> MSSRYRELIAIFGEFLEENDFHVRISMDRVGEVKTLFSAKTIPVESETEAAIEVVTIEAARRRDALRRTCNAVLRTRHSDQHVDVGTIVADEEERLAWKFLIGALAAKNSEILPVVEAELLLAAVEYHYATARPELCDMFVHLSASEMFFIDGDSLFMAALSPQSVDWDLIQPLHVIYNAQKLLYDMHCRGARFHVVFFDSLLWIWESAPAKLFMRENLRKTLMSLSENDAKVGLSISNFSSYYSEAFETYVKQWEPEFILMSDGEQLGRLNPLQAFFVRPSAANNTHDSRRKANYTDADEANPYRLRRQYRSIVEDEAVGDKAALYYRCIHLWAATRRLKVAYSSRIIYKENAMVVFTVRVDGASFERAVTIESDVQALAQSMEHEVQLPAISSASLGLLDEEDLSCRERVVYAALHAYLRASARSEQEHQLCQALAITTYITGYLNKEARAQQVRPNPILAGFLNEISPFLLAVWRHADCTNGNGQEFDLIDGHLFSAVSQQLRTASVSELFDEYGVEDIESTWGVLDDQGSADIVNAPLSYLPVIDSVDVEKLQPYPLITHELVERLAKGFGISTHRADAPYPTDFGAANELAGWDITTPFDRLNDVIDAEGDAIAKSMMTEKEAKNVQEYYKKFVRNALKQAQSMGISGFAAHELAMVCSDNDSDDDAGGNSANNKTAGAKKVNKEHAGQRNKKERSKEDEIRERSNVIAATATVAEWHKQMNHLLHAVDMSHGRTTNRDRDESINTIMAAIKRLSQEKFGKNFDPGYTLGGSTNTAVPLKLEMWRLLVAASQLREVEFAFAMEDPALKDSKGASKKKDSKSEYKMLYGFHVINQFVEREAVKGNHWGQLDPLRKAKPDMTIVEARSYLRWVYLSFVEMHIQLKLKCRVVKLQLENWRAERERARLAQESPKIALGIPLFLYCHHHVLAVIRDEGPRMSSEDIDTVRSALKHFDLPDSYYNKLDQCIARWQNMTLGTLLPSLLPQDKQLFETPEMLQLIHMGHLLERPFVREHDYRVAFNPDNWQRELLDIVDGRGSAVVCAPTSAGKTFISYYCMYKALRRTNKKVVVYLAPARALINQAVADVCARYGSKKYKNPGRYIYGALGGADYHQFHDSCQVLLTVPETFETMLLSPKYTDWVELIDYVILDEIHSMESNGNGDVWERILALLPCPFVALSATLGETQQLCSWLNRVQGRLKEQTEEMSGKMRDFEVHLLPSEGKSIQRWNDIKKYIYLPPPGAALTQKKIKAQYNNCYIRDLHPLSILTADQLQRGFPPDISLVPSEVVSLFEKMHSKFNEVVWPNYSSLQLAKTLRAQLMLIEPSKYFEAETYITQERARQYEAEVKNAFAYWAYLGHEGCELPENLVEEDLDDFSASMNMAVESILRTFAQKLNEDEALLERHAADGMEKKKRMLLRQQHLQLLQQQEQENEPNQEESMEQKSEEQGGAQEEEQEKETVGSVSFPGSRQFIREHILNVLRELIARDMGPTIVFSFESEDCGDLVKYVVEQLEEAESRYRKTNEFALYKARIERAAAAQEARRKQRESTLKQKRLTTGDDGDVEVADRDMSDGEGEDELFVVPDVLPEFTFIGEKCTVEPEVVDSLMEDCEKEGEDLLLRALQRGIGMHHAGVKGKLRAHVERLFRGRHCGVIFSTETLALGIHSPCRSVVLAGDHILLNPTQFRQMMGRAGRRGLDYLGHLVFLGITMRRIKRLMTSSMTVIKGNVQMDPISNLRLLQLYDFNTLRHLKNEAGWKTHVLKLAERLFVNPLFFQGRNSVAGGNMEGFTVEWLQMLLGYFQREGLHFSDHASSLGSILQDAMYVFREAHVGNEGFSFIRMLTSGVFDKAHYSPLYDKKLNSGVLDEPLAELLAYLFS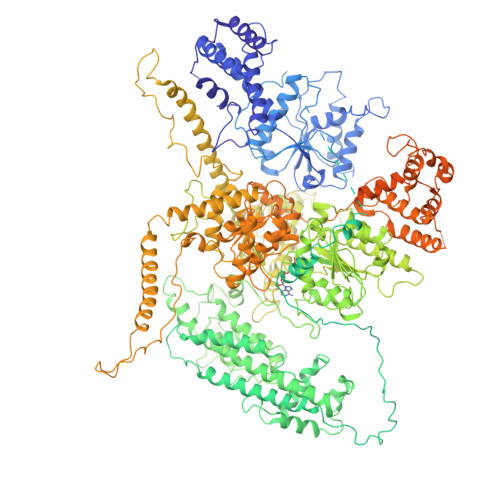THQTCGVPLEMHRSALLDPAVSTLWEGKTGPTQHRAVLSPIDVCSPTIHAFDNTDFFALLSAFYNYLASHLAPQTGAALRLPCMKSTNKKCRIFGGGSTEFLLKQKLQESSVPYKARSPFVAISGCGDLFTSVDDVTFTLRDGLYCDRTLLPILDLADGWRHDGAQILINACLLDFLRAKAQIDTTRKNYRFTLLEELNGLSQSLSYAVLNRAEKILSNLAGLVRPTKLPRAKVLTAIMPDESEEGIFMAGAPRLLEVAERLNSLQPQIQKRLAEELLTAKWAKRISEMNAQRKD3,4-DIMETHYLPHENOL 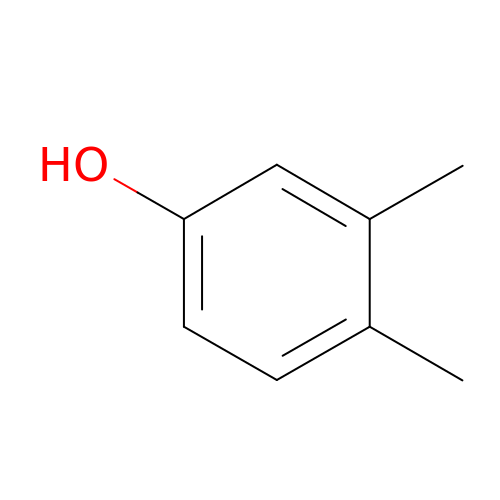| C8 H10 O | YCOXTKKNXUZSKD-UHFFFAOYSA-N2-GUANIDINO-4-METHYL-PENTANOIC ACID [2-(4-{5-[4-(4-ACETYLAMINO-BENZYLOXY)-2,3-DICHLORO-PHENYL]-2-METHYL-2H-PYRAZOL-3-YL}-PIPERIDIN-1-YL)-2-OXO-ETHYL]-AMIDE 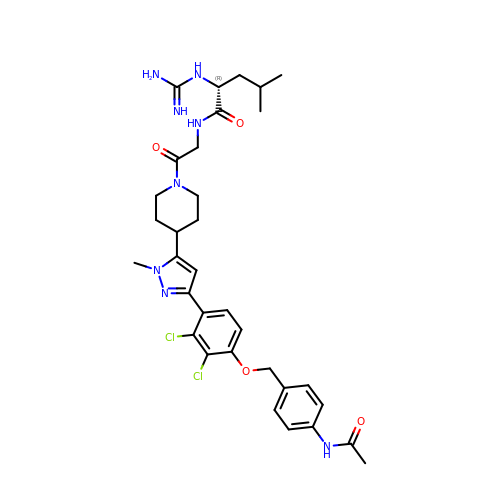| C33 H42 Cl2 N8 O4 | VCXMTWSYQSVWRK-AREMUKBSSA-N> MQEITVDEFSNIRENPVTPWNPEPSAPVIDPTAYIDPQASVIGEVTIGANVMVSPMASIRSDEGMPIFVGDRSNVQ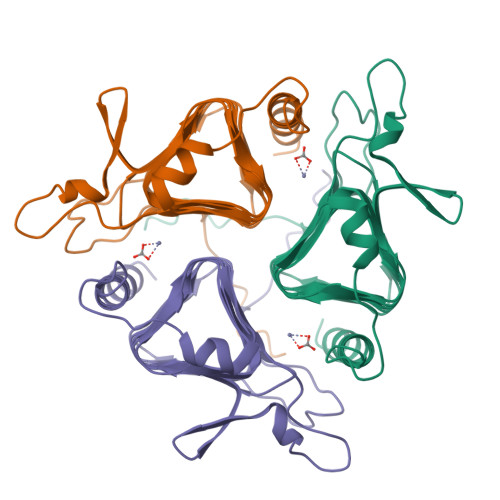DGVVLHALETINEEGEPIEDNIVEVDGKEYAVYIGNNVSLAHQSQVHGPAAVGDDTFIGMQAFVFKSKVGNNCVLEPRSAAIGVTIPDGRYIPAGMVVTSQAEADKLPEVTDDYAYSHTNEAVVYVNVHLAEGYKETS>[2x]ELDGDQMISHRELWAKIANSINDINEQYLKVYEHAVSSYTQMYQDFSAVLSSLAGWI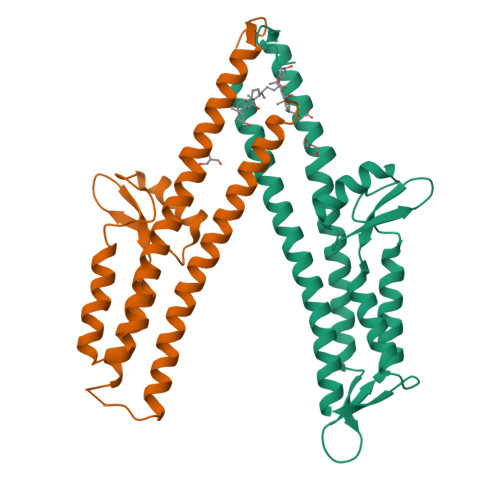SPGGNDGNSVKLQVNSLKKALEELKEKYKDKPLYPANNTVSQEQANKWLTELGGTIGKVSQKNGGYVVSINMTPIDNMLKSLDNLGGNGEVVLDNAKYQAWNAGFSAEDETMKNNLQTLVQKYSNANSIFDNLVKVLSSTIS> MFQTSGLFGQASTTTGGGLFGTAVTPTSTGGSGLFGTSTSIAPTSTGGGLFGTSTAVTPTSTGGGGLFGTSTAVAPTSTGGGGLFGGGGGGGLTSSIGPQGGGGLFGSTTLPTSTSGSGLFGGQSSIGFGQPNSGSGSVSGGLFGSTSVQQPQQQQQQPQQPLITESTKFSDLPPQLKNELQILNKMIINNNSLMNSFSNYDTKINEISIGLDQVASVMDNLFNNFDIHIQSFKYLEESLAKPLNSVNEQVHLLSTQFHSPFSQARPSKEMEIIVDSLVEKIDRIKQTILCVTPTNKSQSQNLSFQESFISTLQSNQIILRNLAYIVDNLVTELERHKKHFLLYKKKYYNQNYNPFLKQPKLNEKTDYHGSSSLHHSHFSQSSNLLSSQSSLFGSSMYGRQSQQQQQQQNPQQSQYLQSSTFQPIQTSTSFFNPTSTTTTTSFGLTNNNNNNNSLASNNSSGGSSGSSLGSLGSLGSGSGSGLFGSTATNNSLGSTSSSGSTSSSIGGSNSIVIPPLAIGSITNNNSGGGLFGSSNSSSNSLN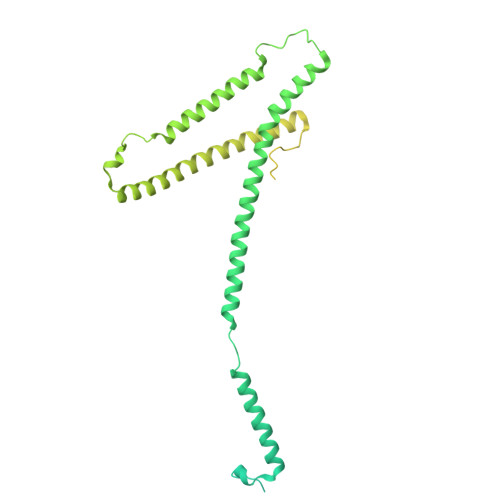SLSTSSSNLFGPPQTPTLSGQGSTLGSVVFQSLVQLQI>MAHHHHHHMEYWHYVETTSSGQPLLREGEKDIFID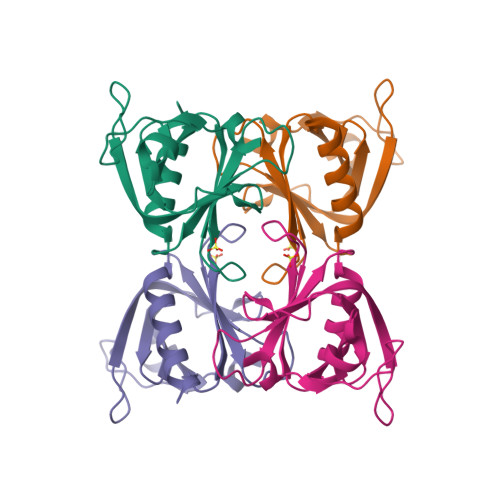QSVGLYHGKSKILQRQRGRIFLTSQRIIYIDDAKPTQNSLGLELDDLAYVNYSSGFLTRSPRLILFFKDPSSSTEFVQLSFRKSDGVLFSQATERALENILTEKNKHIFN[2x]2,5-BIS(4-GUANYLPHENYL)FURAN | C18 H18 N4 O | 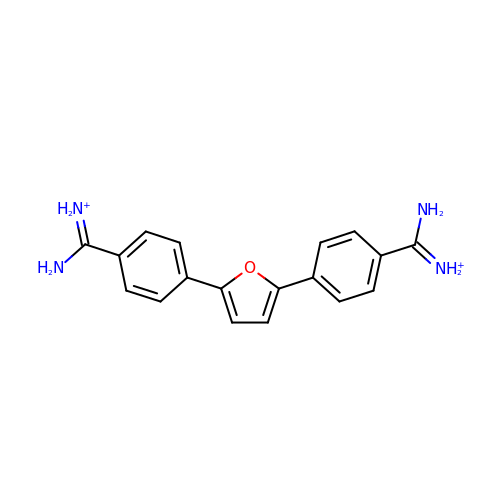ZJHZBDRZEZEDGB-UHFFFAOYSA-P>[2x]GPLGSMTVKLDFEECLKDSPRFRASIELV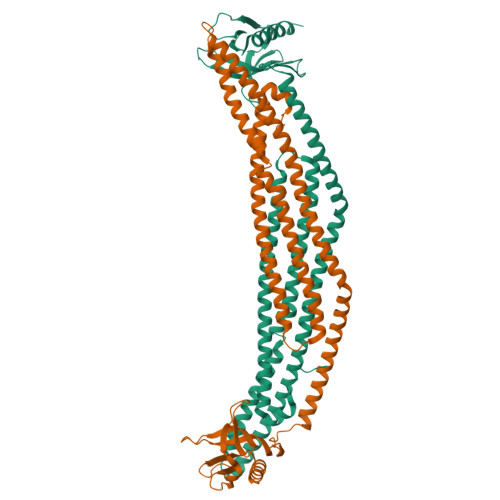EAEVSELETRLEKLLKLGTGLLESGRHYLAASRAFVVGICDLARLGPPEPMMAECLEKFTVSLNHKLDSHAELLDATQHTLQQQIQTLVKEGLRGFREARRDFWRGAESLEAALTHNAEVPRRRAQEAEEAGAALRTARAGYRGRALDYALQINVIEDKRKFDIMEFVLRLVEAQATHFQQGHEELSRLSQYRKELGAQLHQLVLNSAREKRDMEQRHVLLKQKELGGEEPEPSLREGPGGLVMEGHLFKRASNAFKTWSRRWFTIQSNQLVYQKKYKDPVTVVVDDLRLCTVKLCPDSERRFCFEVVSTSKSCLLQADSERLLQLWVSAVQSSIASAFSQARLDDSPRGPGQ(2~{S},3~{S},4~{R})-2-[[4-[4-[2-[2-(2-azanylidenehydrazinyl)ethoxy]ethoxy]phenyl]-1,2,3-triazol-1-yl]methyl]pyrrolidine-3,4-diol 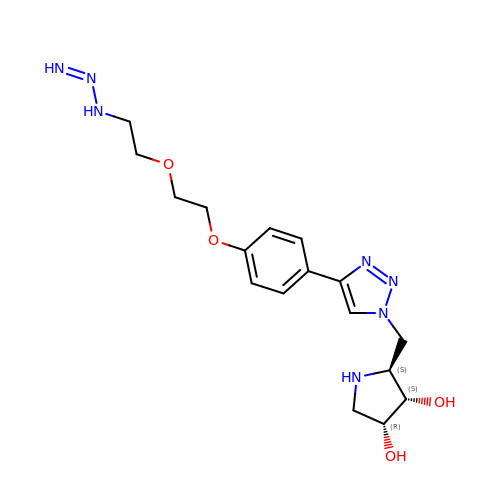| C17 H25 N7 O4 | WVTAXSQMBJVQAL-BBWFWOEESA-N>[2x]FACKTANGTAIPIGGGSANVYVNLAPVVNVGQNLVVDLSTQIFCHN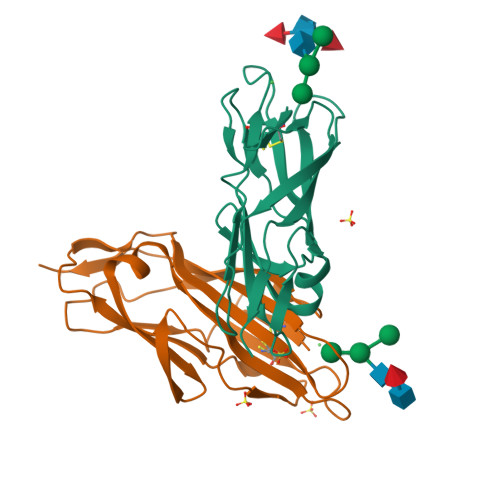DYPETITDYVTLQRGSAYGGVLSNFSGTVKYSGSSYPFPTTSETPRVVYNSRTDKPWPVALYLTPVSSAGGVAIKAGSLIAVLILRQTNNYNSDDFQFVWNIYANNDVVVPT> FDHSGMSVMDRSEGLSISRDGNDLVSVPDQYGWRTARSDVCIKEGMTYWEVEVIRGGNKKFADGVNNKENADDSVDEVQSGIYEKMHKQVNDTPHLRFGVCRREASLEAPVGFDVYGYGIRDISLESIHEGKLNCVLENGSPLKEGDKIGFLLSLPSIHTQIKQAKEFTKRRIFALNSHMDTMNEPWREDAENGPSRKKLKQETTNKEFQRALLEDIEYNDVVRDQIAIRYKNQLFFEATDYVKTTKPEYYSSDKRERQDYYQLEDSYLAIFQNGKYLGKAFENLKPLLPPFSELQYNEKFYLGYWQHGEARDESNDKNT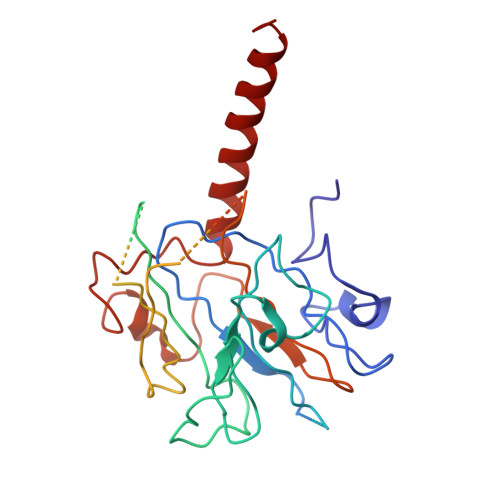TSAKKKKQQQKKKKGLILRNKYVNNNKLGYYPTISCFNGGTARIISEEDKLEYLDQIRSAYCVDGNSKVNTLDTLYKEQIAEDIVWDIIDELEQIAL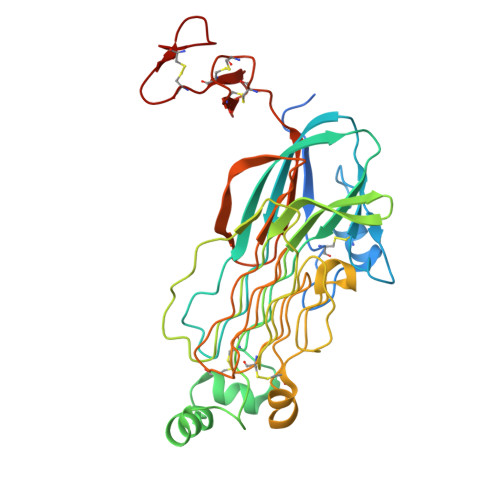> GTAPKSRNLFERNPNKELKPGENSPRQTPIFDPTVHWLFTTCGASGPHGPTQAQCNNAYQNSNLSVEVGSEGPLKGIQIWKVPATDTYSISGYGAAGGKGGKNTMMRSHGVSVLGIFNLEKDDMLYILVGQQGEDACPSTNQLIQKVCIGENNVIEEEIRVNRSVHEWAGGGGGGGGATYVFKMKDGVPVPLIIAAGGGGRAYGAKTDTFHPERLENNSSVLGLNGNSGAAGGGGGWNDNTSLLWAGKSLQEGATGGHSCPQAMKKWGWETRGGFGGGGGGCSSGGGGGGYIGGNAASNNDPEMDGEDGVSFISPLGILYTPALKVMEGHGEVNIKHYLNCSHCEVDECHMDPESHKVICFCDHGTVLAEDGVSCIVSP> MATPASAPDTRALVADFVGYKLRQKGYVSGAGPGEGPAADPLGQALRAIGDEFETRFRRTFSDLAAQLHVTPGSAQQRFTQVSDELFQGGPNWGRLVAFFVFGAALCAESVNKEMEPLV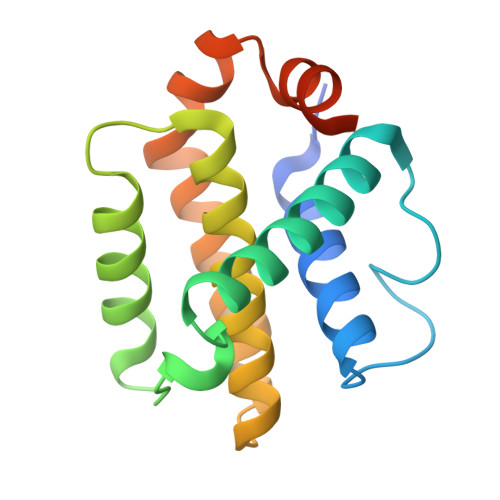GQVQEWMVEYLETRLADWIHSSGGWAEFTALYGDGALEEARRLR>VEGRFQLVAPYEPQGDQPQAIAKLVDGLRRGVKHQTLLGATGTGKTFTISNVIAQVNKPTLVIAHNKTLAGQLYSELKEFFPHNAVEYFVCYYDYYQPEAYVPQTDTYIEKDAKINDEIDKLRHSATSALFERRDVIIVASVSSIYGLGSPEEYRELVVSLRVGMEIERNALLRRLVDIQYDRNDIDFRRGTFRVRGDVVEIFPASRDEHSIRVEFFGDEIERIREVDALTGEVLGEREHVAIFPASHFVTREEKMRLAIQNIEQELEERLAELRAQGKLLEAQRLEQRTRYDLEMMREMGFSSGIENYSRHLALRPPGSTPYTLLDYFPDDFLIIVDESHVTLPQLRGMYNGDRARKQVLVDHGFRLPSALDNRPLTFEEFEQKINQIIYVSATPGPYELEHSPGVVEQIIRPTGLLDPTIDVRPTKGQIDDLIGEIRERVERNERTLVTTLTKKMAEDLTDYLKEAGIKVAYLHSEIKTLERIEIIRDLRLGKYDVLVGINLLREGLDIPEVSLVAILDADKEGFLRSERSLIQTIGRAARNANGHVIMYADTITKSMEIAIQETKRRRAIQEEYNRKHGIVPRTVKKEIR[3x]

Within this complex, UvrA acts as the initial damage sensor but hands off the lesion-containing DNA to UvrB and dissociates, leaving UvrB bound to the lesion in a preincision complex, the precise nature of which is not known. Both UvrA and UvrB expend ATP to form the preincision complex, which is believed to require threading of a β-hairpin element on UvrB through the DNA duplex. UvrB presents the lesion-containing strand to UvrC, which catalyzes hydrolysis of the 5th phosphodiester bond 3′ to the lesion and then the 8th phosphodiester bond 5′ to the lesion. UvrB is classified as a member of SF2 helicases on the basis of conserved helicase motifs (I-VI) (Supplementary ).

If the UvrB helicase domain underwent rigid-body movements similar to those seen for other helicases as proposed previously, ATP-dependent domain closure would force the F-loop toward DNA, perhaps causing F527 to intercalate into the duplex stack, which may function as a “ratchet” to facilitate unidirectional translocation upon ATP-hydrolysis. Indeed, in a structure we determined of UvrB (S91C) bound to a fully base-paired DNA duplex, F527 is intercalated into a sharply bent DNA duplex; furthermore, the crystal structure of the analogous complex containing a F527A mutation revealed substantially reduced DNA bending (Supplementary ) and increased DNA disorder presumably due to the loss of “ratchet” that seems to lock the duplex DNA in position. That F527 intercalation is important functionally suggested by the reduced incision efficiency observed for the F527A mutant UvrB.>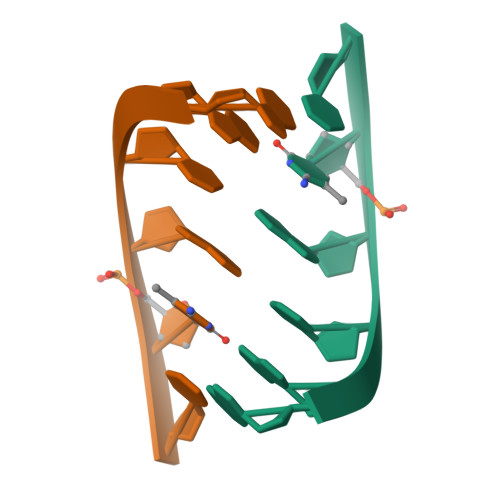[6x]GGCGCC> MEFKLQELNLTNQDTGPYGITVSDKGKVWITQHKANMISCINLDGKI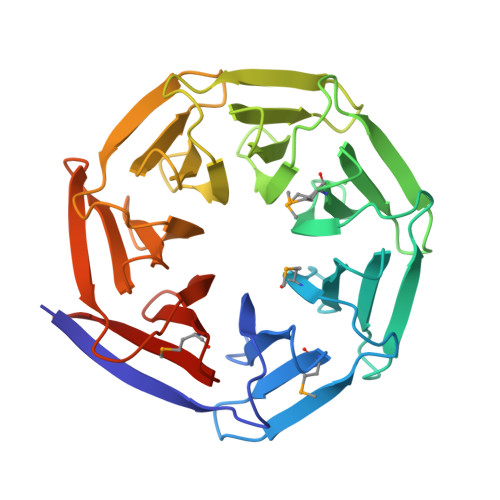TEYPLPTPDAKVMCLTISSDGEVWFTENAANKIGRITKKGIIKEYTLPNPDSAPYGITEGPNGDIWFTEMNGNRIGRITDDGKIREYELPNKGSYPSFITLGSDNALWFTENQNNAIGRITESGDITEFKIPTPASGPVGITKGNDDALWFVEIIGNKIGRITTSGEITEFKIPTPNARPHAITAGAGIDLWFTEWGANKIGRLTSNNIIEEYPIQIKSAEPHGICFDGETIWFAMECDKIGKLTLIKDNME Transcription initiation in bacteria involves the recruitment of RNAP by sigma factors (σ) to promoter regions located upstream from the transcription start site (TSS, position +1). In approximately 60% of bacteria, a major variant σ factor, σ54, forms a class of its own, lacking structural and sequence similarity to σ70. In σ54-mediated transcription initiation, σ54 recruits RNAP to genes responsible for regulating a variety of stress responses, including nutrient depletion, membrane stress, antibiotic exposure, and biofilm formation. In this study, we used single-particle cryo-electron microscopy (cryoEM) to determine the structures of initial transcribing complexes of increasing RNA lengths from 5 nt to 9 nt, which allow us to propose a mechanism of RNAP promoter escape in the σ54 system.

The RII-finger conformation is almost identical between 6 and 5 nt and indeed RNA remains short of reaching RII-finger. In RPitc-6nt and RPitc-7nt, the template strand (at −5 and −6 positions) is scrunched around the RII-finger and σ54 ELH, while the nontemplate strand scrunches around the ELH, resulting in poorly defined density. The ELH density becomes significantly poorer at 6 nt compared to that of 5 nt, indicating that there is an increased flexibility of ELH from 6nt. Up to 6 nt RNA, the upstream DNA remains stably bound to the RNAP-σ holoenzyme. With increasing RNA length (from 6 nt), the enlarged transcription bubble releases the interactions between the bubble and ELH, enabling it to eventually retrieve out of the transcription bubble.

>[2x]SVTEFLKPRLVDIEQVSSTHAKVTLEPLERGFGHTLGNALRRILLSSMPGCAVTEVEIDGVLHEYSTKEGVQEDILEILLNLKGLAVRVQGKDEVILTLNKSGIGPVTAADITHDGDVEIVKPQHVICHLTDENASISMRIKVQRGRGYVPASTRIHSEEDERPIGRLLVDACYSPVERIAYNVEAARVEQRTDLDKLVIEMETNGTIDPEEAIRRAATILAEQLEAFVDLRDVRQPEVKEEKPEFDPILLRPVDDLELTVRSANCLKAEAIHYIGDLVQRTEVELLKTPNLGKKSLTEIKDVLASRGLSLGMRLENWPPA;> MVYSYTEKKRIRKDFGKRPQVLDVPYLLSIQLDSFQKFIEQDPEGQYGLEAAFRSVFPIQSYSGNSELQYVSYRLGEPVFDVQECQIRGVTYSAPLRVKLRLVIYEREAPEGTVKDIKEQEVYMGEIPLMTDNGTFVINGTERVIVSQLHRSPGVFFDSDKGKTHSSGKVLYNARIIPYRGSWLDFEFDPKDNLFVRIDRRRKLPATIILRALNYTTEQILDLFFEKVIFEIRDNKLQMELVPERLRGETASFDIEANGKVYVEKGRRITARHIRQLEKDDVKLIEVPVEYIAGKVVAKDYIDESTGELICAANMELSLDLLAKLSQSGHKRIETLFTNDLDHGPYISETLRVDPTNDRLSALVEIYRMMRPGEPPTREAAESLFENLFFSEDRYDLSAVGRMKFNRSLLREEIEGSGILSKDDIIDVMKKLIDIRNGKGEVDDIDHLGNRRIRSVGEMAENQFRVGLVRVERAVKERLSLGDLDTLMPQDMINAKPISAAVKEFFGSSQLSQFMDQNNPLSEITHKRRISALGPGGLTRERAGFEVRDVHPTHYGRVCPIETPEGPNIGLINSLSVYAQTNEYGFLETPYRKVTDGVVTDEIHYLSAIEEGNYVIAQANSNLDEEGHFVEDLVTCRSKGESSLFSRDQVDYMDVSTQQVVSVGASLIPFLEHDDANRALMGANMQRQAVPTLRADKPLVGTGMERAVAVDSGVTAVAKRGGVVQYVDASRIVIKVNEDEMYPGEAGIDIYNLTKYTRSNQNTCINQMPCVSLGEPVERGDVLADGPSTDLGELALGQNMRVAFMPWNGYNFEDSILVSERVVQEDRFTTIHIQELACVSRDTKLGPEEITADIPNVGEAALSKLDESGIVYIGAEVTGGDILVGKVTPKGETQLTPEEKLLRAIFGEKASDVKDSSLRVPNGVSGTVIDVQVFTRDGVEKDKRALEIEEMQLKQAKKDLSEELQILEAGLFSRIRAVLVAGGVEAEKLDKLPRDRWLELGLTDEEKQNQLEQLAEQYDELKHEFEKKLEAKRRKITQGDDLAPGVLKIVKVYLAVKRRIQPGDKMAGRHGNKGVISKINPIEDMPYDENGTPVDIVLNPLGVPSRMNIGQILETHLGMAAKGIGDKINAMLKQQQEVAKLREFIQRAYDLGADVRQKVDLSTFSDEEVMRLAENLRKGMPIATPVFDGAKEAEIKELLKLGDLPTSGQIRLYDGRTGEQFERPVTVGYMYMLKLNHLVDDKMHARSTGSYSLVTQQPLGGKAQFGGQRFGEMEVWALEAYGAAYTLQEMLTVKSDDVNGRTKMYKNIVDGNHQMEPGMPESFNVLLKEIRSLGINIELED;> LLKFLKAQTKTEEFDAIKIALASPDMIRSWSFGEVKKPETINYRTFKPERDGLFCARIFGPVKDYECLCGKYKRLKHRGVICEKCGVEVTQTKVRRERMGHIELASPTAHIWFLKSLPSRIGLLLDMPLRDIERVLYFESYVVIEGGMTNLERQQILTEEQYLDALEEFGDEFDAKMGAEAIQALLKSMDLEQECEQLREELNETNSETKRKKLTKRIKLLEAFVQSGNKPEWMILTVLPVLPPDLRPLVPLDGGRFATSDLNDLYRRVINRNNRLKRLLDLAAPDIIVRNEKRMLQEAVDALLDNGRRGRAITGSNKRPLKSLADMIKGKQGRFRQNLLGKRVDYSGRSVITVGPYLRLHQCGLPKKMALELFKPFIYGKLELRGLATTIKAAKKMVEREEAVVWDILDEVIREHPVLLNRAPTLHRLGIQAFEPVLIEGKAIQLHPLVCAAYNADFDGDQMAVHVPLTLEAQLEARALMMSTNNILSPANGEPIIVPSQDVVLGLYYMTRDCVNAKGEGMVLTGPKEAERLYRSGLASLHARVKVRITEYEKDANGELVAKTSLKDTTVGRAILWMIVPKGLPYSIVNQALGKKAISKMLNTCYRILGLKPTVIFADQIMYTGFAYAARSGASVGIDDMVIPEKKHEIISEAEAEVAEIQEQFQSGLVTAGERYNKVIDIWAAANDRVSKAMMDNLQTETVINRDGQEEKQVSFNSIYMMADSGARGSAAQIRQLAGMRGLMAKPDGSIIETPITANFREGLNVLQYFISTHGARKGLADTALKTANSGYLTRRLVDVAQDLVVTEDDCGTHEGIMMTPVIEGGDVKEPLRDRVLGRVTAEDVLKPGTADILVPRNTLLHEQWCDLLEENSVDAVKVRSVVSCDTDFGVCAHCYGRDLARGHIINKGEAIGVIAAQSIGEPGTQLTMRTFHIGGAASRAAAESSIQVKNKGSIKLSNVKSVVNSSGKLVITSRNTELKLIDEFGRTKESYKVPYGAVLAKGDGEQVAGGETVANWDPHTMPVITEVSGFVRFTDMIDGQTITRQTDELTGLSSLVVLDSAERTAGGKDLRPALKIVDAQGNDVLIPGTDMPAQYFLPGKAIVQLEDGVQISSGDTLARIPQESGGTKDITGGLPRVADLFEARRPKEPAILAEISGIVSFGKETKGKRRLVITPVDGSDPYEEMIPKWRQLNVFEGERVERGDVISDGPEAPHDILRLRGVHAVTRYIVNEVQDVYRLQGVKINDKHIEVIVRQMLRKATIVNAGSSDFLEGEQVEYSRVKIANRELEANGKVGATYSRDLLGITKASLATESFISAASFQETTRVLTEAAVAGKRDELRGLKENVIVGRLIPAGTGYAYHQDRMRRRAAG;> ARVTVQDAVEKIGNRFDLVLVAARRARQMQVGGKDPLVPEENDKTTVIALREIEEGLINNQILDVRERQEQQEQ;> TAGTPSGNGVDYQDDELPVYQGETTQSLQDYLMWQVELTPFTDTDRAIATSIVDAVDDTGYLTIQIEDIVDSIGDDEIGLEEVEAVLKRIQRFDPVGVAAKDLRDCLLIQLSQFAKETPWLEEARLIISDHLDLLANHDFRTLMRVTRLKEEVLKEAVNLIQSLDPRPGQSIQTGEPEYVIPDVLVRKVNDRWVVELNSDLQEARWLIKSLESANDTLLRVSRCIVEQQQAFFEQGEEYMKPMVLADIAQAVEMHESTISRVTTQKYLHSPRGIFELKYFFSSHVNTEGGGEASSTAIRALVKKLIAAENPAKPLSDSKLTSMLSEQGIMVARRTVAKYRESLSIPPSNQ>MAEQKSSNGGGGGGDVVINVPVEEASRRSKEMASPESEKGVPFSKSPSPEISKLVGSPNKPPRAPNQNNVGLTQRKSFARSVYSKPKSRFVDPSCPVDTSILEEEVREQLGAGFSFSRASPNNKSNRSVGSPAPVTPSKVVVEKDEDEEIYKKVKLNREMRSKISTLALIESAFFVVILSALVASLTINVLKHHTFWGLEVWKWCVLVMVIFSGMLVTNWFMRLIVFLIETNFLLRRKVLYFVHGLKKSVQVFIWLCLILVAWILLFNHDVKRSPAATKVLKCITRTLISILTGAFFWLVKTLLLKILAANFNVNNFFDRIQDSVFHQYVLQTLSGLPLMEEAERVGREPSTGHLSFATVVKKGTVKEKKVIDMGKVHKMKREKVSAWTMRVLMEAVRTSGLSTISDTLDETAYGEGKEQADREITSEMEALAAAYHVFRNVAQPFFNYIEEEDLLRFMIKEEVDLVFPLFDGAAETGRITRKAFTEWVVKVYTSRRALAHSLNDTKTAVKQLNKLVTAILMVVTVVIWLLLLEVATTEVLLFFSTQLVALAFIIGSTCKNLFESIVFVFVMHPYDVGDRCVV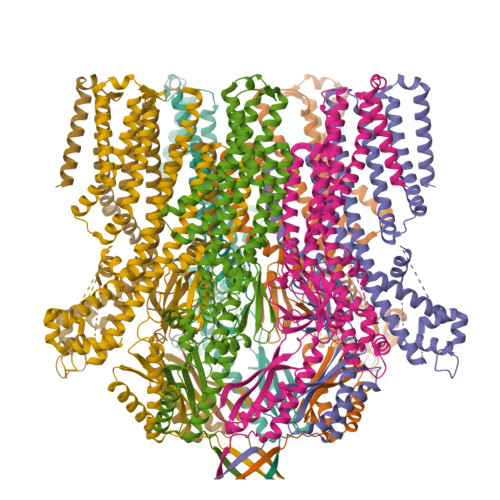DGVAMLVEEMNLLTTVFLKLNNEKVYYPNAVLATKPISNYFRSPNMGETVEFSISFSTPVSKIAHLKERIAEYLEQNPQHWAPVHSVVVKEIENMNKLKMALYSDHTITFQENRERNLRRTELSLAIKRMLEDLHIDYTLLPQDINLTKKNSLEVLFQ[7x]>[3x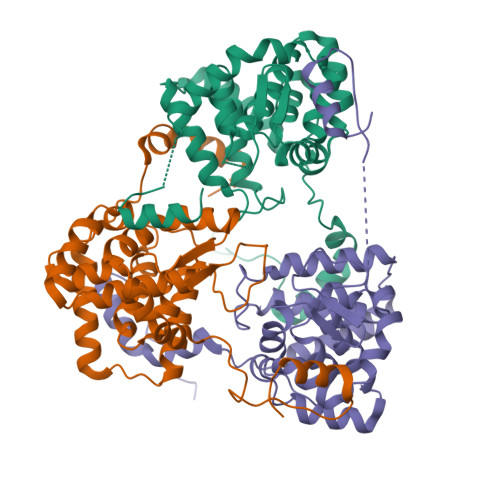]MSKVKLTKENIVALLTQGKDLEFEEDQNLVAFNFKTFCLENLDQIKKMSIISCLTFLKNRQSIMKVIKQSDFTFGKITIKKTSDRIGATDMTFAALDSLIRVRLVEETGNSENLNTIKSKIASHPLIQAYGLPLDDAKSVRLAIMLGGSLPLIASVDSFEMISVVLAIYQDAKYKDLGIDQKKYDTREALGKVCTVLKSKAFEMNEDQVKKGKEYAAILSSSNPNAKGSIAMEHYSETLNKFYEMFGVKKQAKLAELA>[2x]MSNVPHKSSLPEGIRPGTVLRIRGLVPPNASRFHVNLLCGEEQGSDAALHFNPRLDTSEVVFNSKEQGSWGREERGPGVPFQRGQPFEVLIIASDDGFKAVVGDAQ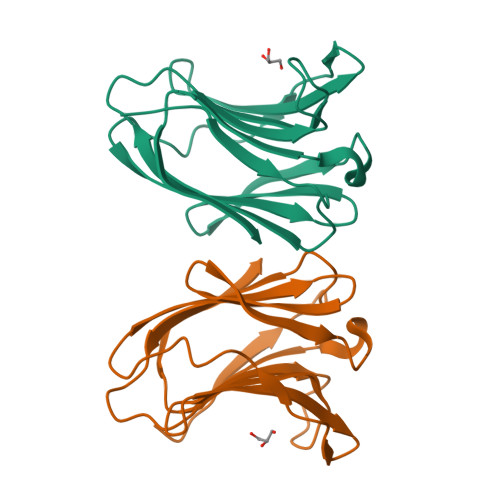YHHFRHRLPLARVRLVEVGGDVQLDSVRIF> MTRQEELAAARAALHDLMTGKRVATVQKDGRRVEFTATSVSDLKKYIAELEVQTGMTQRRRGPAGFY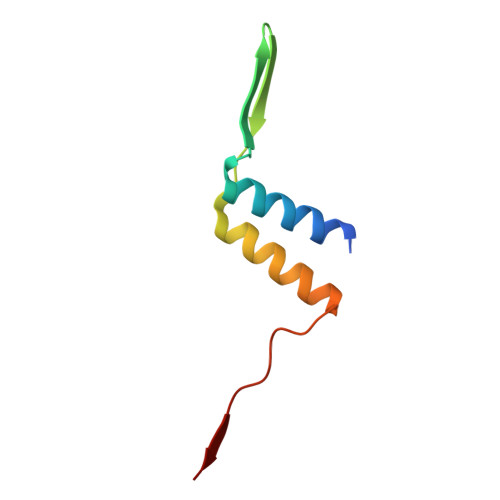V>MHHHHHHSSGRENLYFQGPEQPFIVLGQEEYGEHHSSIMHCRVDCSGRRVASLDVDGVIKVWSFNPIMQTKASSISKSPLLSLEWATKRDRLLLLGSGVGTVRLYDTEAKKNLCEININDNMPRILSLACSPNGASFVCSAAAPSLTSQVPGRLLLWDTKTMKQQLQFSLDPEPIAINCTAFNHNGNLLVTGAADGVIRLFDMQQHECAMSWRAHYGEVYSVEFSYDENTVYSIGEDGKFIQWNIHKSGLKVSEYSLPSDATGPFVLSGYSGYKQVQVPRGRLFAFDSEGNYMLTCSATGGVIYKLGGDEKVLESCLSLGGHRAPVVTVDWSTAMDCGTCLTA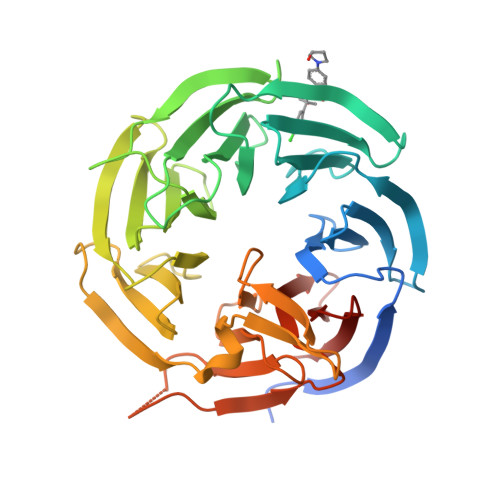SMDGKIKLTTLLAHKA[3x]> GUGUGCCCGGCAUGGGUGCAGUCUAUAGGGUGAGAGUCCCGAACUGUGAAGGCAGAAGUAACAGUUAGCCUAACGCAAGGGUGUCCGUGGCGACAUGGAAUCUGAAGGAAGCGGACGGCAAACCUUCGGUCUGAGGAACACGAACUUCAUAUGAGGCUAGGUAUCAAUGGAUGAGU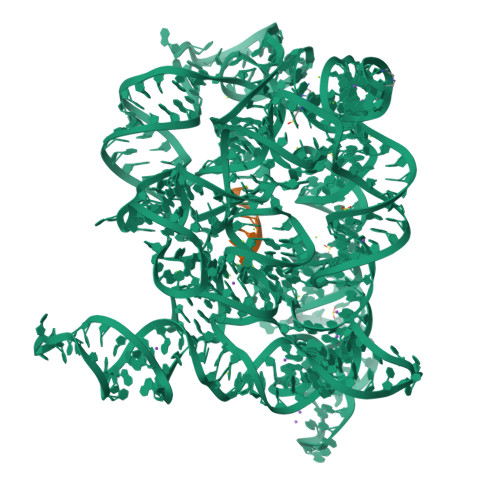UUGCAUAACAAAACAAAGUCCUUUCUGCCAAAGUUGGUACAGAGUAAAUGAAGCAGAUUGAUGAAGGGAAAGACUGCAUUCUUACCCGGGGAGGUCUGGAAACAGAAGUCAGGAGAAGUCAUAGUACCCUGUUCGCAGGGGAAGGACGGAACAAGUAUGGCGUUCGCGCCUAAGCUUGAACGGCCGUAUACCGAACGGUACGUACGGUCGUGUG;> GGGGUUAU> IPNYEFKLGKI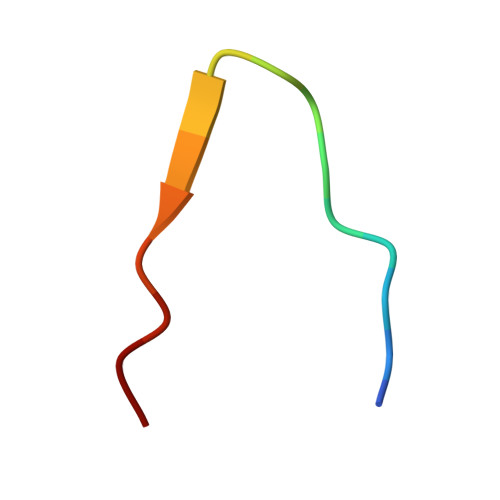TFIRN1-(carboxymethyl)-1H-benzo[g]indole-2-carboxylic acid | C15 H11 N O4 | 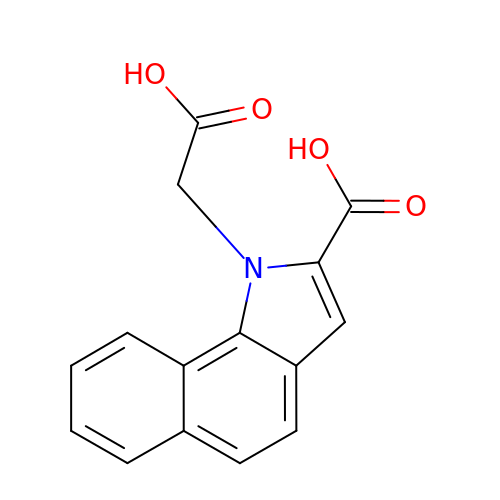AKGLRHRNGGDMDM-UHFFFAOYSA-N>[2x]GAMVDISNPETIRRASSSMSVNVLKGDAIKNYALSEKQYIPFFGSSELSRISPFHPSVLAEKYQRNYRPFLLGAPGTQSLSQYMMMRSAGDAMKNKKVVFIISPQWFVKNGVKTDYFNTYYSELQTYDWLFSMKKVTPADRYLARRLLTFSKVKENDTLTAILQTIKKGKLPLPESLNQLRSQWNMLKREDEVFSNIGLKDRQQKIDHESKRLPKQYQETELSILANQIG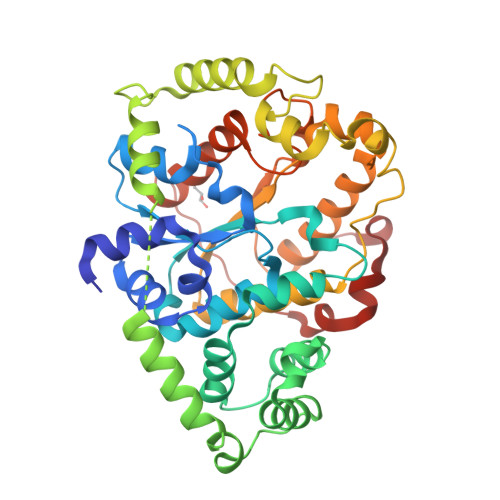ERETTNNPFGLKNDFYTHRIRAHEPELKQSQKNWDYRFSPEFSDFQLVLDQLAKNHNEVLFIIPPVNEKWSDYTGLSQEMLQGFAKKIKFQLNSQGFNRIADFVNQAGTNYFMEDTIHLGWKGWLAADQQIRPFLEENHITASKYHLDDAFFSKSWQHQIPDKLQLK>[2x]MGSSHHHHHHSQDPNSMLSVGATTTATRLTGWGRTAPSVANVLRTPDAEMIVKAVARVAESGGGRGAIARGLGRSYGDNAQNGGGLVIDMTPLNTIHSIDADTKLVDIDAGVNLDQLMKAALPFGLWVPVLPGTRQVTVGGAIACDIHGKNHHSAGSFGNHVRSMDLLTADGEIRHLTPTGEDAELFWATVGGNGLTGIIMRATIEMTPTSTAYFIADGDVTASLDETIALHSDGSEARYTYSSAWFDAISAPPKLGRAAVSRGRLATVEQLPAKLRSEPLKFDAPQLLTLPDVFPNGLANKYTFGPIGELWYRKSGTYRGKVQNLTQFYHPLDMFGEWNRAYGPAGFLQYQFVIPTEAVDEFKKIIGVIQASGHYSFLNVFKLFGPRNQAPLSFPIPGWNICVDFPIKDGLGKFVSELDRRVLEFGGRLYTAKDSRTTAETFHAMYPRVDEWISVRRKVDPLRVFASDMARRLELL

Mtb Decaprenylphosphoryl‐β‐d‐ribofuranose 2‐oxidase (DprE1) is a flavin adenine dinucleotide (FAD)‐dependent enzyme, which together with decaprenylphosphoryl‐d‐2‐ketoerythropentose reductase (DprE2), converts decaprenylphosphoryl‐beta‐d‐ribose (DPR) to decaprenylphosphoryl‐beta‐d‐arabinofuranose (DPA), an essential cell wall component. Multiple covalent3 and non‐covalent4 DprE1 inhibitors have been identified and showed in vitro and in vivo activities against Mtb, further validating DprE1 as an attractive anti‐tuberculosis (TB) drug target. When analyzing toxicity profiles, we noticed that many TCA1 analogs show inhibition of CYP2C9, one of six major cytochrome P450 enzymes which determine the clearance of 75 % of marketed drugs. Here we report the X‐ray crystal structures of WT DprE1, a TCA1‐resistant DprE1 mutant, and CYP2C9 in complex with TCA1 analogs.

Modification of the carbamate group was carried out; however, most of the analogs such as amides and esters are not active, demonstrating the importance of hydrogen bonding between Ser228 and the carbamate group (3.0 to 3.5 Å). When replacing the carbamate with various heterocycles, only TCA020 with pyrimidine showed moderate activity (MIC=2.5 μm, IC50=370±133 nm). To help optimizing the pyrimidyl substituent, we crystallized DprE1 in complex with TCA020. The DprE1–TCA1 structure revealed that the two nitrogen atoms of the pyrimidine ring occupy the positions of the two oxygens of the carbamate group as H‐bond acceptors. Based on these structural insights, we introduced a methyl group at 4‐position of the pyrimidine to gain a hydrophobic interaction with W230 (TCA787), which has similar activity to TCA1.>MAKEKARYFTFLLYPESIPSDWELKLETLGVPMAISPLHDKDKSSIKGQKYKKAHYHVLYIAKNPVTADSVRKKIKLLLGEKSLAMVQVVLNVENMYLYLTHESKDAIAKKKHVYDKADIKLINNFDIDRYVTLDVEEKTELFNVVVSLIRAYTLQNIFDLYDFIDENGETYGLTINLVNEVIAGKTGFMKLLFDGAYQRSKRGTKNEER[3x]

RepB is the rolling-circle replication (RCR) initiator protein encoded by the 5541-bp promiscuous plasmid pMV158, originally isolated from Streptococcus agalactiae and involved in antibiotic resistance spread. It provides both an endonuclease function that constitutes the first step of RCR, and a strand-transfer activity that, together with the endonuclease activity, catalyses the replication termination step1. RepB is a 24 kDa polypeptide that purified and crystallised as a hexamer23. The DNA-binding capability as well as the nuclease and strand-transfer activities of RepB reside in its N-terminal origin binding domain (OBD), which belongs to the replication (Rep) class of the HUH endonuclease superfamily.

We provide an experimental X-ray structure for the Ba2+-RepB6 complex and describe, using both experimental and theoretical techniques, the OBD conformational landscape in the RepB hexamer, showing that the protein displays large intrinsic flexibility at the OBDs level, allowing for fluctuations among multiple conformational states. Surprisingly, a symmetry mismatch occurs between the OD ring and the N-terminal origin-binding nuclease domain (OBD): the OD ring has C6, whereas the OBD ring has either a C2 or an approximate C3 symmetry depending on the crystal form. In geometrical terms, this displacement can be described by a rotation around an axis at an angle of approximately 45° to the central C6 axis of the OD ring, which places the OBD at various distances from the central C6 axis. This leads to a total of nine distinct OBD orientations relative to the ODs in the two crystal structures solved, three for the C2 form and six for the C3 form. A structural element that may contribute to stabilize the outward position of the OBD is the presence of a metal ion bound in this area. The coordination of the metal ion is provided by backbone carbonyl oxygen atoms of the 310 helix of the hinge region and the side chain of residue E181 of helix α7 of the same protomer. In addition, E137 (OD helix α5) of an adjacent protomer interacts with the metal ion through a bridging water molecule instead of making a salt bridge with R7, as when the OBD is closer to the C6 axis (inward and intermediate positions). To confirm the metal ion binding, we co-crystallised RepB6 with Ba2+ and exploited the X-ray absorption of the Ba2+ ion. The anomalous difference map shows that the Ba2+ occupies the same position assigned previously to a Mg2+ ion. Some density was also observed in the protomer where the OBD is in an intermediate position, and was refined as a Ba2+ ion with half occupancy. However, the presence of divalent metal ions in the medium does not seem to be determinant in driving the hexamer towards the C2 conformation, as Mg2+ was also used in the crystallization solution of C3 (even though no divalent cation could be located in this structure).N-(2,2,2-TRIFLUOROETHYL)-N-{4-[2,2,2-TRIFLUORO-1-HYDROXY-1-(TRIFLUOROMETHYL)ETHYL]PHENYL}BENZENESULFONAMIDE | C17 H12 F9 N O3 S | 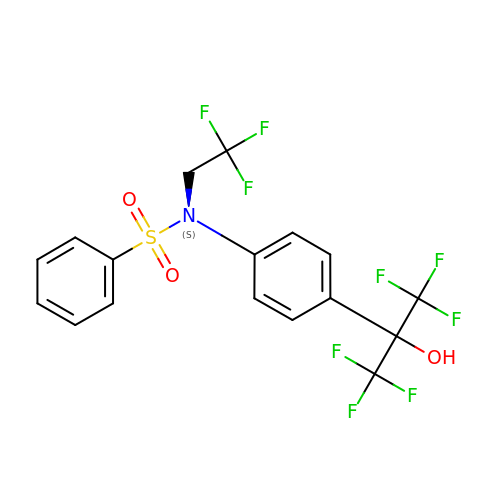SGIWFELWJPNFDH-UHFFFAOYSA-N4-methyl-6-{3-[(methylamino)methyl]phenyl}pyridin-2-amine 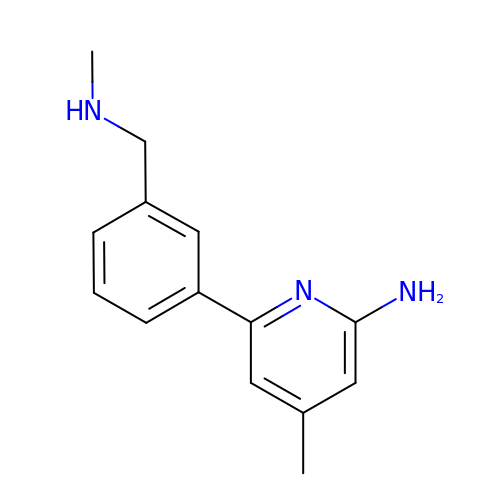| C14 H17 N3 | QVLCJJWOAMFHSP-UHFFFAOYSA-N>[2x]MAKDKEFQVLFVLTILTLISGTI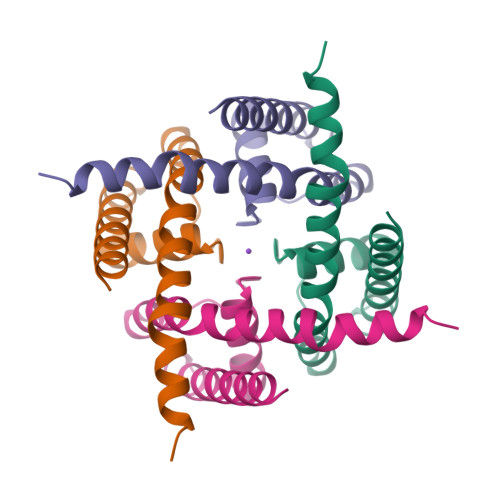FYSTVEGLRPIDALYFSVVTLTTVGYGEFSPQTDFGKIFTILYIFIGIGLVFGFIHKLAVNVQLPSILSNLVPR>GAMERVLKVFHYFENSSEPTTWASIIRHGDATDVRGIIQKIVDCHKVKNVACYGLRLSHLQSEEVHWLHLDMGVSNVREKFELAHPPEEWKYELRIRYLPKGFLNQFTE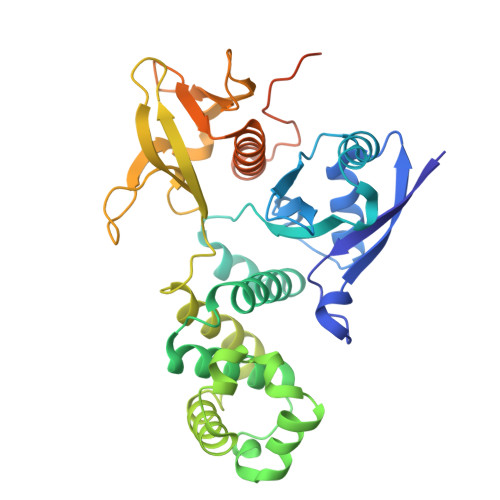DKPTLNFFYQQVKNDYMLEIADQVDQEIALKLGCLEIRRSYGEMRGNALEKKSNYEVLEKDVGLRRFFPKSLLDSVKAKTLRKLIQQTFRQFANLNREESILKFFEILSPVYRFDKECFKCALGSSWIISVELAIGPEEGISYLTDKGANPTHLADFNQVQTIQYSNSEDKDRKGMLQLKIAGAPEPLTVTAPSLTIAENMADLIDGYCRLVNGATQSFIIRPQKEGERALPSIPKLANNEKQGVRSHTVSVSETDDYAE[2x]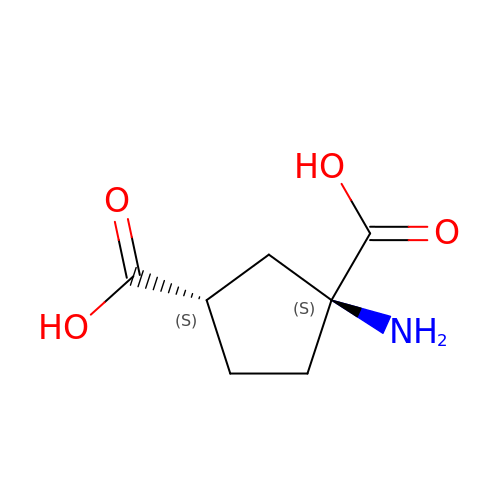(1S,3S)-1-aminocyclopentane-1,3-dicarboxylic acid | C7 H11 N O4 | YFYNOWXBIBKGHB-FFWSUHOLSA-N> RFIPWFP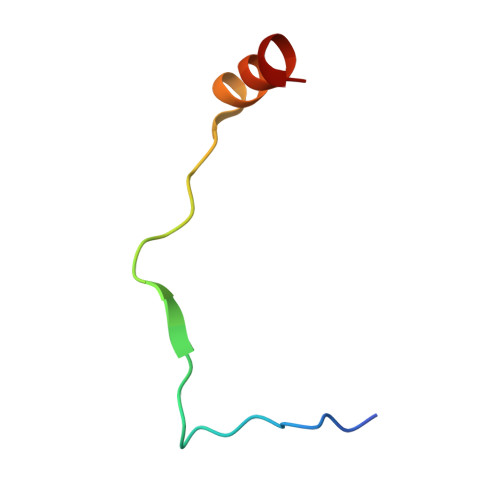YDGSKLPLRPKRSPPVISEEAAEDVKQYLT>FNASSGDSKKIVGVFYKANEYATKNPNFLGCVENALGIRDWLESQGHQYIVTDDKEGPDCELEKHIPDLHVLISTPFHPAYVTAERIKKAKNLKLLLTAGIGSDHIDLQAAAAAGLTVAEVTGSNVVSVAEDELMRILILMRNFVPGYNQVVKGEWNVAGIAYRAYDLEGKTIGTVGAGRIGKLLLQRLKPFGCNLLYHDRLQMAPELEKETGAKFVEDLNEMLPKCDVIVINMPLTEKTRGMFNKELIGKLKKGVLIVNNARGAIMERQA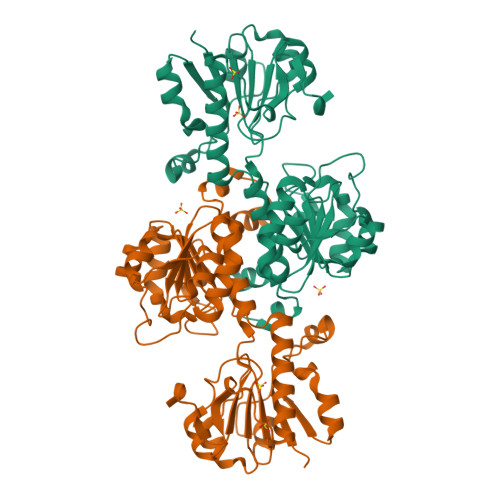VVDAVESGHIGGYSGDVWDPQPAPKDHPWRYMPNQAMTPHTSGTTIDAQLRYAAGTKDMLERYFKGEDFPTENYIVKDGELAPQYR[2x]> APLF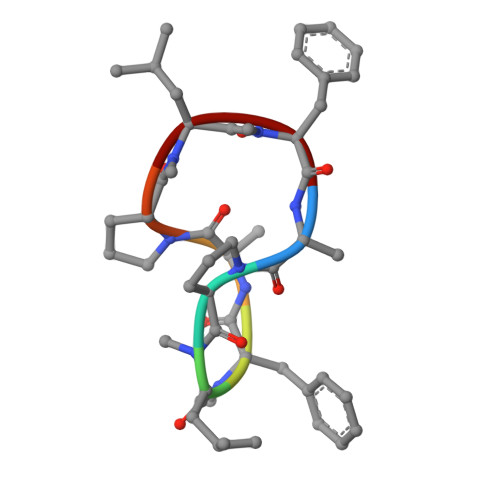APLF> MTFAKIKFSAQIRLETGLHIGGSDAFAAIGAIDSPVIKDPITNLPIIPGSSLKG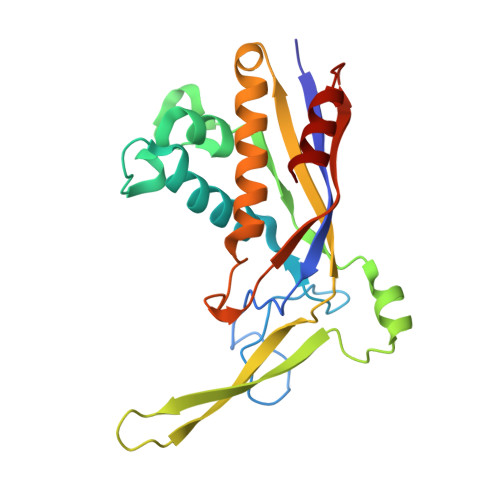KMRTLLAKVYNEKVAEKPSDDSDILSRLFGNSKDKRFKMGRLIFRDAFLSNADELDSLGVRSYTEVKFENTIDRITAEANPRQIERAIRNSTFDFELIYEITDENENQVEEDFKVIRDGLKLLELDYLGGSGSRGYGKVAFENLKATTVFGNYDVKTLNELLTAEV Intramembrane proteases are one class of membrane proteins, which share the property of cleaving transmembrane (TM) proteins to release cytoplasmic, luminal, or extracellular domains that move to new locations where they can carry out their biological functions. Rhomboids, first discovered as part of the epidermal growth factor signalling pathway in Drosophila, are characterised by a core of six TM helices. Structures of the rhomboid protease GlpG from Escherichia coli and Haemophilus influenzae have revealed that the catalytic dyad serine and histidine forms part of a water-filled cavity separated from the external medium by a flexible loop and from the bilayer by TM helices. Substrate proteins are thought to diffuse laterally through gaps between TM helices to reach the rhomboid active site.

The second crystal form of GlpG S201T was obtained by using a lipid detergent mixture, dimyristoyl phosphatidylcholine (DMPC)/3-[(3-cholamidopropyl) dimethylammonio]-2-hydroxy-1-propanesulfonate (CHAPSO), which has a tendency to form bicelles or bilayers. These crystals belonged to the orthorhombic space group P212121 and diffracted to 1.7 Å. A comparison of this structure obtained in a lipid environment with the GlpG S201T in a detergent environment shows major differences only in the loop regions, which are reflected in their temperature factors. The displacement of His254 due to S201T substitution is much more pronounced in the structure determined in a detergent environment than in the structure determined in a lipid environment. The crystals of GlpG S201T obtained by mixing with lipids are type I membrane protein crystals, as described by Michel, which mimic a lipid bilayer. A total of 14 fully or partially ordered lipid molecules have been modelled in the current structure, and with contributions from symmetry-related lipid molecules, they form an annulus around the protein. The presence of connected density for two acyl chains in three of the modelled lipids unambiguously distinguishes them from detergent. Most lipid molecules are clustered around TM1, L1, and TM3 in both leaflets. A well-ordered lipid molecule, PC502, fits nicely into the groove created by helices TM2 and TM5. Second, the bilayer thickness around GlpG varies across the protein, and lipid molecules adapt to match the local environment of the protein.

> AGPVTWVMMIACVVVFIAMQILGDQEVMLWLAWPFDPTLKFEFWRYFTHALMHFSLMHILFNLLWWWYLGGAVEKRLGSGKLIVITLISALLSGYVQQKFSGPWFGGLTGVVYALMGYVWLRGERDPQSGIYLQRGLIIFALIWIVAGWFDLFGMSMANGAHIAGLAVGLAMAFVDSLNA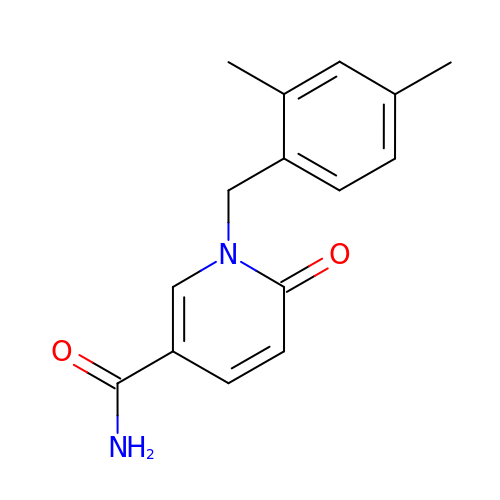1-(2,4-dimethylbenzyl)-6-oxo-1,6-dihydropyridine-3-carboxamide | C15 H16 N2 O2 | TUJVPUNUHQIBSM-UHFFFAOYSA-N>TRFTEEYQLFEELGKGAFSVVRRCVKVLAGQEYAAKIINTKKLSARDHQKLEREARICRLLKHPNIVRLHDSISEEGHHYLIFDLVTGGELFEDIVAREYYSEADASHCIQQILEAVLHCHQMGVVHRNLKPENLLLASKLKGAAVKLADFGLAIEVEGEQQAWFGFAGTPGYLSPEVLRKDPYGKPVDLWAC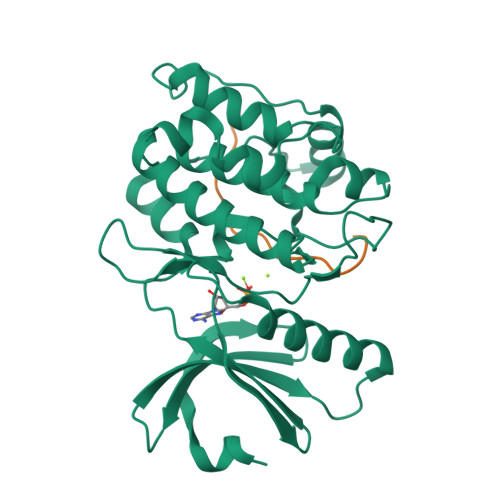GVILYILLVGYPPFWDEDQHRLYKQIKAGAYDFPSPEWDTVTPEAKDLINKMLTINPSKRITAAEALKHPWISHR[2x];>[2x]KAQKKNRNKLRRQHSYDTFVDL>[3x]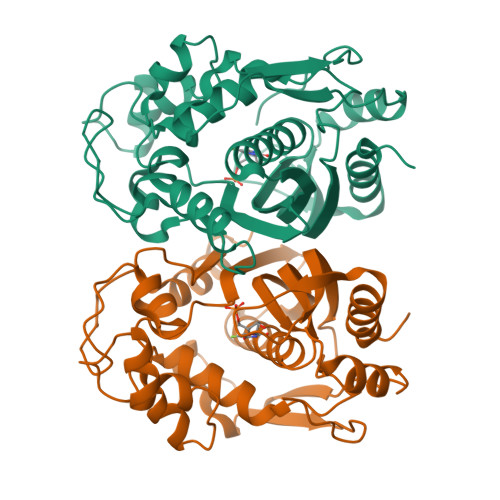MRGSHHHHHHGSMPVAGSELPRRPLPPAAQERDAEPRPPHGELQYLGQIQHILRCGVRKDDRTGTGTLSVFGMQARYSLRDEFPLLTTKRVFWKGVLEELLWFIKGSTNAKELSSKGVKIWDANGSRDFLDSLGFSTREEGDLGPVYGFQWRHFGAEYRDMESDYSGQGVDQLQRVIDTIKTNPDDRRIIMCAWNPRDLPLMALPPCHALCQFYVVNSELSCQLYQRSGDMGLGVPFNIASYALLTYMIAHITGLKPGDFIHTLGDAHIYLNHIEPLKIQLQREPRPFPKLRILRKVEKIDDFKAEDFQIEGYNPHPTIKMEMAV> MKKTLPTKKSNLWFLMACLIITFHKVEAQVPDPNQGLRAEWMRGALGMLWLPERTFNGNIEGIRIDDFLTQIKDIRTVDYVQLPLTSPNIFSPTHVAPHPIIESLWQGDTDANGDPINLVAPRESVDDPLLSWLKALRAAGLRTEIYVNSYNLLARIPEDTQADYPDVSARWMEWCDTNTEAQAFINSQTYHEGNGRRKYMFCYAEFILKEYAQRYGDLIDAWCFDSADNVMEDECGDDPASEDVNDQRIYQAFADACHAGNPNAAIAFNNSVGDREGNPFTSATLFDDYTFGQPFGGAGNMVVPEALYTYNHDLVVFMQTNNGYAFRDDTRTWNDNVVAHFFPKQSTTSWNAGNTPCLTDEQFVEWTSTGIVNGGGITWGTPLVRTNLENAPVLTLQPYALNQFELTDTYLKEFQSPGKPNWSRQYTILPAIYPGQPYSHNLVEGVDFWDPEGVGITGLTASGTLPAWLTISQTATGTWTLSGTPPVSEASNYTFELMAQDSDGVTNREVKLEVISHPAGFTNPGDGTPVWFSNPMVLAKATALKDYGSLLKLGVDFYDFEGDVLTITKTSGPDWLVLTQNSDDTWRLSGMPTAADAGENSFTFNVSDGILSSDTEIKITVDHVAGF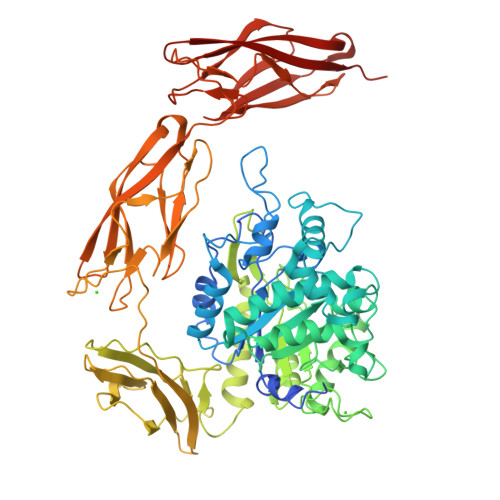TNLGNGAPVWSSPILNLTDGKGSFAYNYTLQLGTDYYDFEGDALTITKTSGPDWLTIQQTDANSWKLSGTPINSDAGENSFTFNLSDDTNSTTAEILINVIATIIS In S. coelicolor A3(2), a total of four proteins CprA, CprB (the coelicolor pigment regulator proteins), ScbR (S. coelicolor QS receptors) and ScbR2, have been identified as GBL receptors. The structure revealed that it belongs to TetR (tetracycline repressor) superfamily of transcriptional regulators (TetR-FTRs) comprising a DNA binding domain (DBD) and a ligand-binding domain (LBD) at the N- and C-terminus of the protein, respectively. The DBD recognizes and interacts with the cognate operator sequence (OS) through the helix-turn-helix (HTH) motif, whereas the LBD regulates the DNA binding activity by interacting with its cognate inducer molecule. CprB consists of 10 α-helices, among which, three of the N-terminal α-helices α1, α2 and α3 form the core DBD, with spacer helix α2 (residues 33–39) and recognition helix α3 (residues 43–49) constituting the signature HTH motif, commonly present among transcription regulators.

The crystal structure of CprB in complex with the CS was determined to a resolution of 3.25 Å. The asymmetric unit of the CprB–CS complex consists of two CprB dimers and a double-stranded DNA. The DNA sequence used for complexation was semi-palindromic (5′-ACATACGGGAC*GCCCCGTTTAT-3′, where the asterisk represents the dyad axis) and has been previously shown by Sugiyama et al. to bind ArpA as well as CprB. In contrast to the apo form of the protein, which is a dimeric unit, the CprB–CS complex was found to be a dimer of dimers. Both the dimeric units are bound at opposite sides of the 22-bp CS and there are no interactions between the two dimers. Comparative analysis of the CprB–CS complex and the apo form of CprB was performed using LBD domain as a reference frame. Binding of the CS to CprB induces a general pendulum-like movement in the overall protein structure as shown in Figure 1C. A twist in the dimeric interface results in a coordinated motion of the DNA binding HTH motif about the connector helix α4. This motion facilitates a snug fit of helix α3 into the major groove of the CS, thereby aiding DNA binding event. The ligand pocket volumes also change from ∼635 Å3 in the apo form to ∼750 Å3 in the DNA-bound form, indicating that the operator-bound form of the dimer is a more open structure with an increased accessibility to the ligand-binding pocket. The average of all the roll and twist angles in the DNA are around 0.9° and 35.5°, respectively, yielding a global bend of ∼3.5° in the DNA as compared to the standard B-form. The CprB–CS complex is stabilized by a total of around 35 phosphate backbone and 20 direct base contacts, shown in Figure 2A and B. The direct base contacts in the monomers are mostly through the residues K43, G44, Y47 and F48, whereas residues H49, Y47, T42, S33, T31 and K53 interact via the phosphate backbone.

>[4x]MARQLRAEQTRATIIGAAADLFDRRGYESTTLSEIVAHAGVTKGALYFHFAAKEDLAHAILEIQSRTSRRLAKDLDGRGYSSLEALMRLTFGMARLCVQGPVLRAGLRLATAGVPVRPPLPHPFTEWREIATSRLLDAVRQSDVHQDIDVDSVAHTLVCSVVGTRVVGGTLEPAGREPRRLAEMWYILIRGMVPVTRRARYVTLAARLEQETGTA> TAPATAADVKQVGYVQQIIGAVVDVTFTDSVPPVLTALTVDAKETGTLLTMEIVQHLDTKTARCICMSSTDMLRLRTPVVNTGSQITVPVGEATLGRIFNVMGDAIDQRG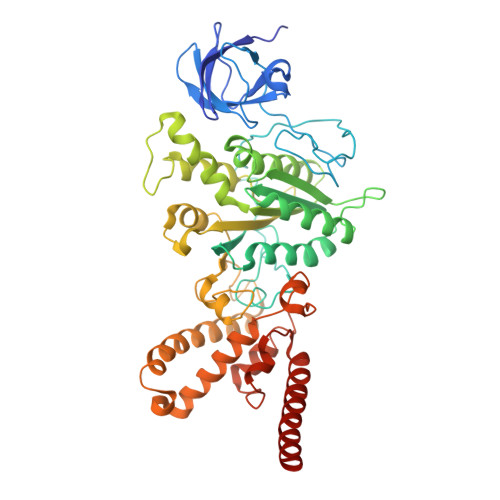PVKNKVRWPIHRKAPTLAEQSGKDEVLVTGIKVIDLILPYCKGGKIGLFGGAGVGKTVIIMELINNVAKGHGGYSVFAGVGERTREGTDLYLEMMGSKVIDLQGDSKCVLVYGQMNEPPGARARVAQTALTMAEYFRDEAGQDVLLFVDNVFRFTQANSEVSALLGRIPAAVGYQPTLAEDLGMLQERITSTVKGSITSVQAVYVPADDITDPAPATTFSHLDATTVLSRSVAEAGIYPAVEPLECASRIMDPDAIDVNHYNVAMDIVEMLTKYKELQDIIAVLGIDELSEEDKLIVDRARKVAKFMSQPFAVAEVFTGMKGYYVQLEDCVSDFGSLLMGQCDNIPEMAFYMVGGLDSVKEKAAKMAAEAAAMRERARKAAEAK> MTEFWLISAPGEKTCQQTWEKLHAATTKNNNLAVSSKFNIPDLKVGTLDVLVGLSDELAKLDAFVEGVVKKVAQYMADVLEDSKDKVQENLLASGVDLVTYITRFQWDMAKYPIKQSLKNISEIIAKGVTQIDNDLKSRASAYNNLKGNLQNLERKNAGSLLTRSLAEIVKKDDFVLDSEYLVTLLVVVPKLNHNDWIKQYETLAEMVVPRSSNVLSEDQDSYLCNVTLFKKAVDDFRHKARENKFIVRDFQYNEEEMRADKEEMNRLSTDKKKQFGPLVRWLKVNFSEAFIAWIHIKALRVFVESVLRYGLPVNFQAMLLQPNKKSVKKLREVLHELYKHLDSSAAAIIDAPMDIPGLNLSQQEYYPYVYYKIDCNLLEFK;>[3x]MALSDADVQKQIKHMMAFIEQEANEKAEEIDAKAEEEFNIEKGRLVQTQRLKIMEYYEKKEKQIEQQKKIQMSNLMNQARLKVLRARDDLITDLLNEAKQRLSKVVKDTTRYQVLLDGLVLQGLYQLLEPRMIVRCRKQDFPLVKAAVQKAIPMYKIATKKDVDVQIDLEAYLPEDIAGGVEIYNGDRKIKVSNTLESRLDLIAQQMMPEVRGALFGANANRKFLD;>[3x]MASQSQGIQQLLQAEKRAAEKVADARKRKARRLKQA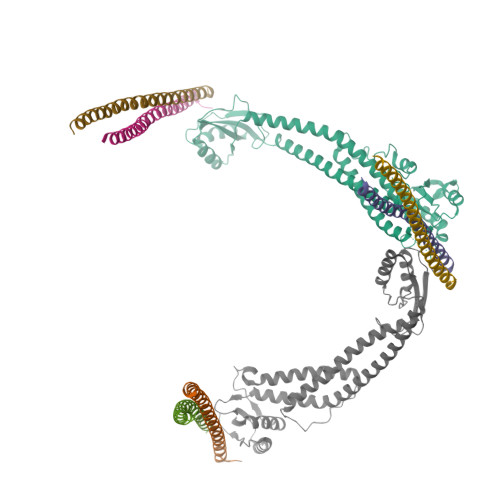KEEAQMEVEQYRREREQEFQSKQQAAMGSQGNLSAEVEQATRRQVQGMQSSQQRNRERVLTQLLGMVCDVRPQVHPNYRITV;> MGELFRSEEMTLAQLFLQSEAAYCCVSELEELGKVQFRDLNPDVNVFQRKFVNEVRRCEEMDRKLRFVEKEIRKANIPIMDTGENPEVPFPRDMIDLEANFEKIENELKEINTNQEALKRNFLELTELKFILRKTQQFFDEMADPDLLEESSSLLEPNEMGRGAPLRLGFVAGVINRERIPTFERMLWRVCRGNVFLRQAEIENPLEDPVTGDYVHKSVFIIFFQGDQLKNRVKKICEGFRASLYPCPETPQERKEMASGVNTRIDDLQMVLNQTEDHRQRVLQAAAKNIRVWFIKVRKMKAIYHTLNLCNIDVTQKCLIAEVWCPVTDLDSIQFALRRGTEHSGSTVPSILNRMQTNQTPPTYNKTNKFTHGFQNIVDAYGIGTYREINPAPYTVITFPFLFAVMFGDFGHGILMTLFAVWMVLRESRILSQKNENEMFSMVFSGRYIILLMGLFSIYTGLIYNDCFSKSLNIFGSSWSVRPMFTIGNWTEETLLGSSVLQLNPAIPGVFGGPYPFGIDPIWNIATNKLTFLNSFKMKMSVILGIIHMLFGVSLSLFNHIYFKKPLNIYFGFIPEIIFMSSLFGYLVILIFYKWTAYDAHSSRNAPSLLIHFINMFLFSYPESGNAMLYSGQKGIQCFLIVVAMLCVPWMLLFKPLILRHQYLRKKHLGTLNFGGIRVGNGPTEEDAEIIQHDQLSTHSEDAEEPTEDEVFDFGDTMVHQAIHTIEYCLGCISNTASYLRLWALSLAHAQLSEVLWTMVIHIGLHVRSLAGGLGLFFIFAAFATLTVAILLIMEGLSAFLHALRLHWVEFQNKFYTGTGFKFLPFSFEHIREGKFDE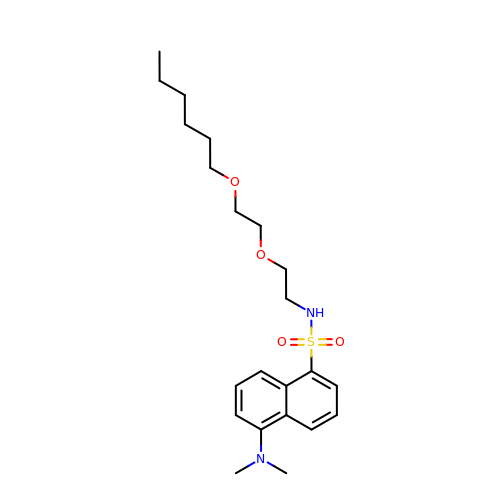5-(dimethylamino)-~{N}-[2-(2-hexoxyethoxy)ethyl]naphthalene-1-sulfonamide | C22 H34 N2 O4 S | ZQDZHRAPTBKCCR-UHFFFAOYSA-N> EPKVYRQREGMIQFVFQWGIGNSFRAVSANRFRPVHAARPKEVSIHPSYFESPHPFVIWEPLNEAWEVYFYENLKKSAKPFPVKKFGI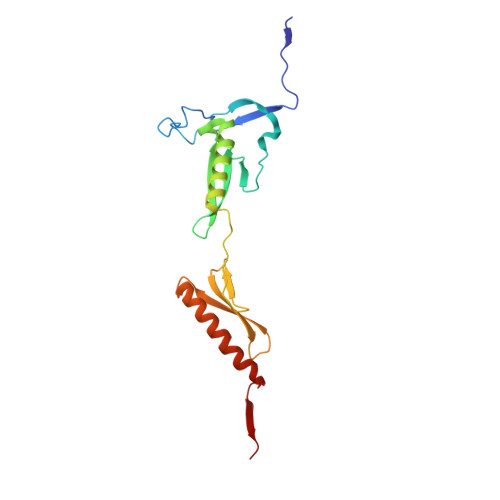ARAKREALLFLEQMKLEGKLEKPTFSSGVDGVTFDQVTGSWICRFVDEEGRCVSRGFGADFHGFEEARKLAIERQAEMKKVEASGLGPRMRLVKEK>[2x]MGSSHHHHHHHSSGLVPRGSHHMLEMQINLPEVHAEVTAQFVRYEKALTSNDTAVLNELFWNSPQTLRYGATENLYGYEAIAGFRATRSPNNLEREIVRTVITTYGHDFATANIEFRRLSHSQLTGRQSQTWMRTSQGWRVVAAHVSLIALPVS

AtzH is the first DUF3225 family protein that has been shown to possess a catabolic function, likely decarboxylating the product of AtzEG-mediated deamination of 1-carboxybiuret as part of the cyanuric acid mineralization pathway. The data presented here imply that AtzH is a decarboxylating, 1,3-dicarboxyurea amidohydrolase. AtzH belongs to NTF2-fold superfamily, which contains 38 protein families, including the AtzH family: DUF3225 (DUF: domain of unknown function). Size exclusion chromatography performed on AtzH after removal of the his-tag, suggested that the native protein had a molecular mass of ~ 29 kDa, consistent with a dimer (2 x 14,655 kDa).

We obtained the X-ray crystal structure of the AtzH. Differential Scanning Fluorimetry (DSF) was used to estimate the stability of the protein and showed that the native protein had a Tm of 57.2°C. Well diffracting crystals of AtzH grew readily, and two different space groups were observed: P1 and C2221. X-ray diffraction data were collected for both. Analysis with PISA gives an interfacial surface area of almost 3,200 Å2 (or about 29% of the total surface area of the protein). The AtzH active site was sought by examining the X-ray structure. However, an in silico docking simulation between the X-ray crystal structure of the AtzH dimer and 1,3-dicarboxyurea elucidated a potential active site. The arginine residues form an extensive hydrogen bonding network with the carbonyl oxygens of 1,3-dicarboxyurea. Tyr22 is positioned within 3 Å of the carbonyl carbon of one of the two terminal carboxylic acids, and Arg46 is within hydrogen-bonding distance of the hydroxyl group of Tyr22. Tyr22 and Arg46 are therefore well positioned to form a catalytic dyad, albeit one of atypical composition.> GPGSMDFAPSARAAELIAAVREFIDAEVMPVERAVLAHHDELLGARAGTTAELWHVPPELDSLKAKARAAGLWNLFLPDPELGGGLSNSEYAPLAEQMGRSLFAPTVFNCNAPDSGNMEVLHRYGSQEQKEVWLEPLLEGDIRSAFCMTEPDVASSDATNMAATAVVEGDEVVINGRKWWSTGVGHPDCKVIIFMGLTDPNAHRYARHSMVLVPMDTPGITVERMLPTMGFYD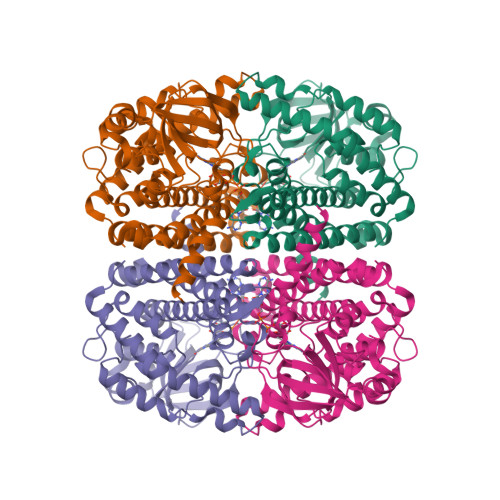EPGGHGVVSFDNVRLPADAFIAGPGKGFEIAQGRLGPGRVHHAMRLIGLAEVALEHACRRGLDRTAFGKPLVNLGGNRERIADARIAINQTRLLVLHAAWLLDTVGIMGALSAVSEIKVAAPNMAQQVIDMAIQIHGGGGLSNDFPLAAAWVNARALRLADGPDEVHRGVVARIELAKYAND> RAGDRLSGAAARGDVQEVRRLLHRELVHPDALNRFGKTALQVMMFGSTAIALELLKQGASPNVQDTSGTSPVHDAARTGFLDTLKVLVEHGADVNVPDGTGALPIHLAVQE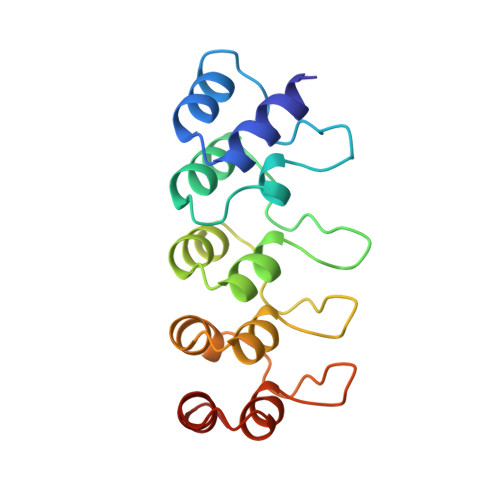GHTAVVSFLAAESDLHRRDARGLTPLELALQRGAQDLVDILQGHM Textilinin-1, isolated from the venom of the Australian brown snake, Pseudonaja textilis, is an experimental drug (Q8008, Venomics Pty Ltd) and is suggested as a novel anti-bleeding agent to replace aprotinin. Textilinin-1 is a good inhibitor of plasmin but with a more narrow binding specificity compared to aprotinin. Kunitz-type inhibitors (similar in structure to aprotinin) are one class of small protein commonly found in such venoms. Herein, we describe a kinetic study of the inhibition of human plasmin and plasma kallikrein by textilinin-1 and aprotinin, and report the crystal structure of the complex between urokinase-activated microplasmin (protease domain of human plasmin) and textilinin-1.

For microplasmin no electron density connects R561 and V562 confirming that the peptide bond between these two residues was, as expected, cleaved by urokinase. The α-amino group of V562 is in the “activated” position making an ionic bond with the side-chain of D740. The hydrogen bonds that stabilize this β-sheet are between P15O of textilinin-1 and G762N of microplasmin and R17N of textilinin-1 and S760O of microplasmin. P15 makes a kink in the structure of textilinin-1, which positions its amide nitrogen too far from the microplasmin surface to form a hydrogen bond. However, this proline is stabilized by hydrophobic contacts to W761 of microplasmin. The most important polar attraction is an interaction between G39O of textilinin-1 and E606OE1 of microplasmin. The side-chain of I36 of textilinin-1 is exposed to the solvent but does form hydrophobic attractions with E687, Q738 and to a lesser extent H603 of microplasmin. Nonetheless, as suggested earlier, the structures of the two complexes show that the interaction between microplasmin and textilinin-1 is flexible and there is freedom of movement around the P1’ site if outside forces such as those due to crystal packing are present. On the other hand, the movement of the histidine side-chain in the complex with textilinin-1 reduces the surface complementarity at this site. The observation that the histidine side-chain is out of its position in the catalytic triad in the microplasmin complex and the flexible nature of the canonical loop in textilinin-1 could not have easily been predicted by molecular modelling.

>SFDCGKPQVEPKKCPGRVVGGCVAHPHSWPWQVSLRTRFGMHFCGGTLISPEWVLTAAHCLEKSPRPSSYKVILGAHQEVNLEPHVQEIEVSRLFLEPTRKDIALLKLSSPAVITDKVIPACLPSPNYVVADRTECFITGWGETQGTFGAGLLKEAQLPVIENKVCNRYEFLNGRVQSTELCAGHLAGGTDSCQGDSGGPLVCFEKDKYILQGVTSWGLGCARPNKPGVYVRVSRFVTWIEGVMRNN[2x];>[2x]KDRPDFCELPADTGPCRVRFPSFYYNPDEKKCLEFIYGGCEGNANNFITKEECESTCAA>[2x]MAFAKELFLGKIKKKEVFPFPEVSQDELNEINQFLGPVEKFFTEEVDSRKIDQEGKIPDETLEKLKSLGLFGLQVPEEYGGLGFSNTMYSRLGEIISMDGSITVTLAAHQAIGLKGIILAGTEEQKAKYLPKLASGEHIAAFCLTEPASGSDAASIRSRATLSEDKKHYILNGSKVWITNGGLANIFTVFAKTEVVDSDGSVKDKITAFIVERDFGGVTNGKPEDKLGIRGSNTCEVHFENTKIPVENILGEVGDGFKVAMNILNSGRFSMGSVVAGLLKRLIEMTAEYACTRKQFNKRLSEFGLIQEKFALMAQKAYVMESMTYLTAGMLDQPGFPDCSIEAAMVKVFSSEAAWQCVSEALQILGGLGYTRDYPYERILRDTRILLIFEGTNEILRMYIALTGLQHAGRILTTRIHELKQAKVSTVMDTVGRRLRDSLGRTVDLGLTGNHGVVHPSLADSANKFEENTYCFGRTVETLLLRFGKTIMEEQLVLKRVANILINLYGMTAVLSRASRSIRIGLRNHDHEVLLANTFCVEAYLQNLFSLSQLDKYAPENLDEQIKKVSQQILEKRAYICAHPLDRTCHHHHHH;>[2x]MGQDPVELAMFGLRHMEPDLSARVTIYQVPLPKDSTGAADPPQPHIVGIQSPDQQAALARHNPARPVFVEGPFSLWLRNKCVYYHILRADLLPPEEREVEETPEEWNLYYPMQLDLEYVRSGWDNYEFDINEVEEGPVFAMCMAGAHDQATMAKWIQGLQETNPTLAQIPVVFRLAGSTRELQTSSAGLEEPPLPEDHQEEDDNLQRQQQGQSLEHHHHHH

The Mitochondrial Complex I Assembly (MCIA) complex is essential for the biogenesis of respiratory Complex I (CI), the first enzyme in the respiratory chain, which has been linked to Alzheimer’s disease (AD) pathogenesis. Here we report the structural basis of the complex formation between the MCIA subunits ECSIT and ACAD9. ECSIT binding induces a major conformational change in the FAD-binding loop of ACAD9, releasing the FAD cofactor and converting ACAD9 from a fatty acid β-oxidation (FAO) enzyme to a CI assembly factor. The inclusion of an additional N-terminal 26 residues in the ECSIT construct (hereafter named ECSITCTER, residues 221–431), combined with optimisation of the purification and subcomplex reconstitution protocols led to a 3.0 Å resolution cryo-EM structure of the ACAD9WT-ECSITCTER complex, enabling us to build and refine an atomic model that includes nearly all ACAD9 residues as well as a 15-residue peptide spanning ECSIT residues 320–334. As previously described, ACAD9 is present as a dimer, where the C-terminal regions (residues 600–621) form helix loops that are positioned around the neighbouring protomer thereby stabilising the active dimer.

The ECSIT binding site is located at the junction of the ACAD9 dehydrogenase and vestigial domains, with one ECSITCTER per ACAD9 protomer. ECSIT residues 322–328 form a 310-helix that interacts with the ACAD9 β1–β2 loop, while ECSIT residues 329–334 adopt an extended loop conformation lying in anti-parallel orientation between the ACAD9 α16 and η6 helices. Specifically, ECSIT Glu323 makes a salt bridge with ACAD9 Lys228, stabilising the ECSIT binding on the N-terminal segment with the ACAD9 β4 strand, whereas a second salt bridge between ECSIT Asp333 and ACAD9 Arg446 stabilises the ECSIT binding on the C-terminal end with the ACAD9 α16 helix. Furthermore, ECSIT directly interacts with the ACAD9 β1–β2 loop through three hydrogen bonds between ECSIT Trp324 and ACAD9 Ser191 and Asp188, respectively, and ECSIT Glu323 with the backbone amide of Ile192. Notably, while there is no evidence of direct ECSIT interactions with the second ACAD9 protomer, Asp188 shows an additional hydrogen bond with Asn333 on α11’–α12’ loop, bridging ECSIT binding with the ACAD9 dimer. Examination of the electrostatics properties of the binding interface shows that the surface of the ACAD9 is mainly positively charged whereas the modelled ECSIT sequence is mostly negative. In contrast, the loop adopts a very different conformation in the ACAD9WT-ECSITCTER model, where the tip of the β1-β2 loop (residue Gly186) moves by ~10 Å upwards to allow the ECSIT 310-helix to insert, suggesting that this mobile ACAD9 β1-β2 loop plays the role of a gatekeeper. Thr320 forms hydrogen bonds with Gln331, stabilising the helical sequence that enters into the ACAD9 binding cavity.> MATEGGGKEMNEIKTQFTTREGLYKLLPHSEYSRPNRVPFNSQGSNPVRVSFVNLNDQSGNGDRLCFNVGRELYFYIYKGVRKAADLSKPIDK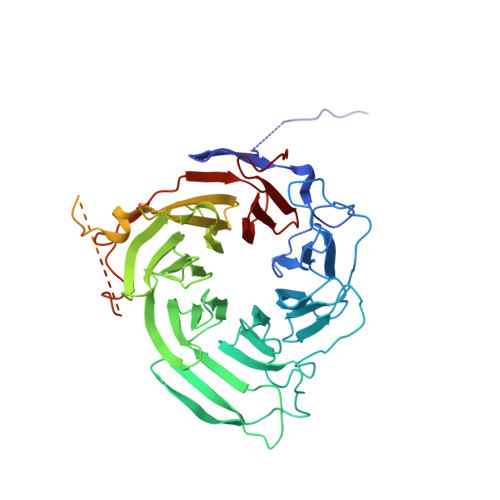RIYKGTQPTCHDFNHLTATAESVSLLVGFSAGQVQLIDPIKKETSKLFNEERLIDKSRVTCVKWVPGSESLFLVAHSSGNMYLYNVEHTCGTTAPHYQLLKQGESFAVHTCKSKSTRNPLLKWTVGEGALNEFAFSPDGKFLACVSQDGFLRVFNFDSVELHGTMKSYFGGLLCVCWSPDGKYIVTGGEDDLVTVWSFVDCRVIARGHGHKSWVSVVAFDPYTTSVEEGDPMEFSGSDEDFQDLLHFGRDRANSTQSRLSKRNSTDSRPVSVTYRFGSVGQDTQLCLWDLTEDILFPHQPLSRARTHTNVMNATSPPAGSNGNSVTTPGNSVPPPLPRSNSLPHSAVSNAGSKSSVMDGAIASGVSKFATLSLHDRKERHHEKDHKRNHSMGHISSKSSDKLNLVTKTKTDPAKTLGTPLCPRMEDVPLLEPLICKKIAHERLTVLIFLEDCIVTACQEGFICTWGRPGKVVSFNP> SWKVKEIVIMSVISIVFAVVYLLFTHFGNVLAGMFGPIAYEPIYGIWFIVSVIAAYMIRKPGAALVSEIIAALVECLLGNPSGPMVIVIGIVQGLGAEAVFLATRWKAYSLPVLMLAGMGSSVASFIYDLFVSGYAAYSPGYLLIMLVIRLISGALLAGLLGKAVSDSLAYTGVLNGMALGKELKKKRKRASEHASL

Energy coupling factor (ECF) transporters form a large superfamily of prokaryotic membrane translocation systems involved in the uptake of scarce nutrients and trace elements from the environment. They form a modular complex consisting of two integral transmembrane proteins, a T component, and an S component that form the conduit for the substrate, coupled to a soluble ATP-binding cassette (ABC) protein (Rodionov et al., 2009). The S component is involved in substrate recognition and generally interacts with its substrate molecule with very high affinity (Duurkens et al., 2007, Erkens and Slotboom, 2010). The yko operon encodes for a group I ECF module, where YkoE acts as the substrate-capture S component, YkoC as the T component and YkoD represents the ABC component consisting of two fused ATPase domains.

We determined the structure of a thiamine-bound group I substrate-capture (S) component (YkoE), an integral membrane protein that is part of a dedicated tripartite transporter complex, in a lipidic environment. The structure was solved using single-wavelength anomalous dispersion (SAD) with selenomethionine-labeled YkoE to 1.95 Å resolution. The structure of YkoE revealed a six helical transmembrane domain with the overall fold reminiscent of S components from group II ECF transporters (root-mean-square deviation between YkoE and other S components ranges between 2.6 and 3.6 Å). YkoE possesses an additional C-terminal helix that presumably protrudes toward the cytosol and lies perpendicular to the lipid bilayer. The six hydrophobic helices form a tight fold with an open cavity with a volume of 545 Å3 facing the extracellular part of the membrane. The thiamine molecule is present at the base of the cavity found in the extracellular part of the membrane. The pyrimidine group forms π-stacking interactions with a highly conserved Trp49 located at the kink of helix H2. In addition, the pyrimidine group is coordinated by H bonds by highly conserved Glu77 and Gln95 residues located on helix H3 and H4, respectively. The thiazole ring of thiamine forms H-bonding interactions with Asp131 and Tyr46. The thiamine-binding crevice in YkoE is open and not protected by lid closure mediated by loop L1 as observed for several group II ECF S components (Zhang et al., 2010, Erkens et al., 2011, Zhao et al., 2015).(2S)-2-[(8S,9S,10R,13S,14S,17R)-10,13-dimethyl-3-oxo-2,3,6,7,8,9,10,11,12,13,14,15,16,17-tetradecahydro-1H-cyclopenta[a]phenanthren-17-yl]propanoic 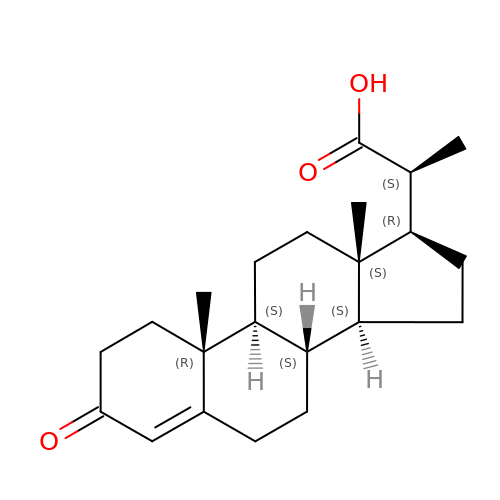acid (non-preferred name) | C22 H32 O3 | QETBTXOVEBTJQH-WAMTXRNCSA-N> MFLIHFVHYKTILQKYTFKFKHIFLSIDKYNSLFFNISGILIWLNIIHINIILIKYSFFILINNFEYLIILIST;> MQKLLSPRTARHARLFRLAGKLADSGSPGVPKSDGERLVWVNSHVRRDKDISLSQEEERIRELMMPLEVGENSFAANGQATHGNLFYFREYPMYPGEYVPAEHNTLSSLRDELRLDLTAQSLKEAWMRVSGGVYFQSVDEYYASVDGLDAEQIGEVLAALFPELNCYEAQALVQRTLECISRPVSAASRQLSRTITAEAVGLDNAPGHYTNFLEWMGRLTETRAFKTEHALFEFSRRKFNRDDVRVMFENYRLMSKATLLADSADSYSHFYTVLKDFAXKVAGEDSRHQIGVRIDEAEVDPETGIAVGRGCADGEKYHFTALLRENRDHNGIITVMGKPLSLVLDNKAWLMEMVLMPFDEANLDYRDFDAHIVSEGHAMPSIANEIAAFALRMAVANALVKLIPLTRIPLKKSGLLSVDRRRERGQFPGYLDGKKVKRRFAKR;> MVRRSHVVAYYWSRYRMPTQMPKFDGPAPVAAPQSMNSTKTNEFIDPIDDKFPMSIRGPLVRPDVPEDQYVDSWYICTSMTHHMGDYRPWSASAPPNAFRFRPFNEFDAKGREYVQYMREFARFDPRKSRGNGQKGFPFRDAYLTKMNEANQKTPPPTLETIMDRAVREHHQHARILSPLEVQRDVGRLEPIPSYAGKINADRSVFPFQWKTEDWYEYEVAKVRNRRFVFENTEEDGIRGSEVTYKIVLEGFWDHHVMKLAEDVCMFLKDVGRQIVEEKLVAVRRLLQGGAVDPELLAAFNCARAGPFGGLDEYDKEEVANFLRSDLRRLEEQCLSVINRCNVPVPGATNIYDPHTSWPHVEKLEPWVRMAEFWTSSSDTSFTELEMSTAHYEFRKFFRVIICKLPFQSTEFEKRMYDIRHWLHRQTSCEFHTIYRRNVIHDSAVFPTEHDPATPTTHEHHRMFSFALDWQSAPVNRLSTDTVHEGESWDAVAQRLGCSVGELKDANAERETIEAGVVINVPVTATRRLTSFGATPLVLPLKTTSAKDGERIRTWEEAAAILDCTVEELQQCNGHAALTYQKKESEAGEFDSSETELVAPLSCWTSTSESEFSPVERVHANDTLVAIARRLQCSEEALRAVNDGITDVSGLDFVRVPPEARRPRRLVEPQLRPQAATDALLARTIAEEETFKLKSIPHLPQNAERFPHEYHTPTSRFPPTPSETPATQDWMAYTAKYLDKQFTISAEPAPVYNVNKLWPMQQIPGKVDQTPFEEDQTWLLHSIPVQQLEMHHHEKDLQDLPFINHEQFPRSLEWNAP;> MMRKSVTFLRRGKPRPRAGMFPDKYRRVPMLLKPQQGGQQYFNHFLIRSTNDRLTQQDVDNASGQAHSFISPQLPQMDWRNMSARSSEESIREEMRQLAENDVMQHQRVFNERMWYEKEEEHRMKARSCPEETSEHAXSNDGAVPPPRVLGGDYFKTRFGYSLVKNSEMTQGPVDYSQLDMWGEMPRYTSDMVFLYLVSRRRNTYAVAYTYEGKRILNTYTAGNRGLKGGDRGFRSEGSTDNGHQVTSMYLNDLLPKLREMRASEGRPMGRGEKVELVVRVMGFYNGRQGAVRAVQDRANEFHVRYFEDITPFPLNGPKMPRGVFK;> MFCFSRGLWMRHIGQDVPKRHTHFVLESRLMYEKSFRDCWLHSVCRAISQLDEPLSKTVVGTHQKMLQRKVTCFQYNQYGLFKTPYYRLANVDRYHAVQGVAGTREWVPYVNVSYWTMNKMVRGGNLLVHRVHYTGWGTDSHLKKGGWEHRWNKVLQRNVLQYSRI;> MNRTGGSIYAHALSQFAVCRQPWNEYIGLLTKQDSTPYHTEPQEKPAYRGRK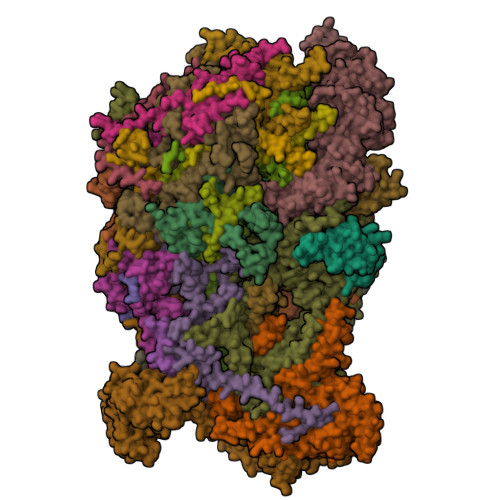QGREGWLFGQQVQLHYHRFPDEQLITNLSRWRTGETVGDIAMQQFRNAQPFDIEDKDPQGVQRPSPEVYMKLNYKNPATISRFLTRTGHMYPADILPLNPEAVVKLRVAKAQAIRIGLYPRFGNPFWFRSQKFRPKAYQENYDPTTYSTKRTVEHFAYNWVQTDRIRRYFRELEAVHTSGSASARGSGGGTTAEHKQQDQFYSPENQPISLHRNNISYMEDVGRSVKNPTVPGLMSTKGMKKKFHNLYSSTSTKRMGFSNPTLGIKKV;> MAFRNTFTTPGKFSTVSKNIVLLLIWRVKVFLRAEGFAHSLVMLPVSLYSKILLCDVKKKIVYFHCCTRKKSMLRRCPCVWPDGPTKSSVSIGTAFTLQKRFLKIAKSAFGFYLARRGQRKYPFLRRPHIKNTHSMNPSAPYFWSFMTAKSQMAFLPEENYITGDWTGKFFVSKRQVYTLQHATSGAKVRVKSFPSIFEFNSPSRWNIGKEMNTLTKPRMDLIDEQMLTKKQRLDYVRAGLLPK;> MRSKTLKKSLAAMYMRPPVTCYTDACEAPVAMWDGAIPLKETRKLKNGVPVRTVSRTYSHPPQLTPTQLSFNDINSMYCVGNDELIQFFPEGLGGRVFQTMPPGHPRGFLYRKETHLLNLFVDKVQHWHTKRSVLSSLTNGRTGFIVDGPTGCGKSALMCQVVHFARSRNIVTLYVPDAKVWTHGEWCWPSTILPGFFDAPDAARSFLKYFAVANRATLTSWKLRCTPKDLPTEQGERQPQNLYELCEWGHRAVAPASIDRQSVCVKFLMDELSEEKKLPVVIVVDGWNLFSHETHFRYPHPDFLRGLASFNESSTDIDLYPQELPRIPASRLSFVRGLNKMILSGDDPNKFFITCTTRDFKPFDGISGFPNVETDRFANSLDEYAPYDPEKDSHFHPIQIGNFDEYEYRSFLRFLINSGELAGLGWGPLWHASSDFERKLYKIGFLSGRNPQGVVDHYHQELVWRYDYQRTRQKQYLLKRRMEGMSRGASSGAVGVR;> MVLRRWFPLLGVHRVGYTHPSTLPVPCAQRWDLRLARARIFQEYIEEKAPGAWQLEDERSMSPEFKTFTGYPMRDMRPGYGQNLPDYIMKKRLPNNTHYELFARRDIPNEDNAMYGKYLYDMTVHGTSLPSTYRMHKDINKAQRNDRKLSGNRFKVLCSSGAKNPPSGWEPIPDATEEEED;> MRRWHRSLNPALFGERGSGHYFSTTRARLQLQAQDRIICGTHGAGIVAHQTAVNSSDNPMLSSVTTAAPAADLSRTKPHEGTGTSERDPYIRTLHNQRSAAPESSVSQSHTVNAPTVDECEMLAERWGTMNYWHNDTFPRLVVFLKKLLVPDVSPLSPTAESLLSMFEKVVIPKLTSDEEDRRKLVSLWSETTLQAEAAVTKFLFQRGSFESMLHRIITDALEKMSTLALGGQEGNLALEALKRQTLFKRNDYIQKRLIDVVSNSAYLGYGDSVWQVFFAAVEANEENLLSDRATTDAIRAAWEGVMREDVVRLPDVTGVVALYLTLVCIRESGRLVPEELKELSSGLEDGVRPGVRKLQQYPLIFLHPTVKRRFVVKAVAEILHNSSSNAFSNMLRENGLHDTAREVALCEAMNRNKELAEGDVGDAVGRFVSKGEVKTLLSSLVSGTDAVVRDAVAGIFGIGTTITIDWDAVMQNVDWSNNWQRLATALLSNSAVLSAIVKLVKNAIGAKGMSKHLFTDEYADQLQLILDAREERAASRKQRIENIAQELSSFERVDLSCDLLRKLGVDMTELDTAAAATRNMNVVQRPCIEDGLLSLVLEAVTKRHPNWVKAGVIQTTLKDPFDALRWMMHIFIRLSYVPHAGAATIARLSRRRIGPIGLEPHQFNVPAELGFVEQYDNLQYKRYDWQGWYQRMLDVHNRNVSLRCRICDLQRLDGNGVQFVDMQTERRLRILAQHRVGMGVLKLDADKYEDQADNVTFGTTKLSELLADARKAQLGEEYWPSVELKVRKPSGQSKAHYSLIDNERIEKRSRELYEKYRDAKKRSLFVTPMETWLEVKGMQVRKSVDNADEDGYTLDALQDMMDGDDGDKV;> MMRRVASTGSNGGHCYVGSSLWADSVYMEVSSITLQKRFSFKYATKLQHDEMRQPYYIHEKRYGIFSNERNIAKARRGLPFITPLYTKHMNLWDTDTDASNNRFFRGYYYGQRELHQLLGRPHSLEATNADGSNDLSTYEANTSQLYKGIPRPAITNLHYEPAWRYTLYQAGAHGAQLSNPRSPFTAKVLGDELMQVRDIKSVEHCKAWFDRLQYLINLHYEAVGDIGEFKSRHTRHVHEFFVAFHDALSSLDFRDTYLFDQFKAVRPPELSDLFGIFLEMEANYVHEDYCPRCSLPYSTTRYCGEGDVDTPFRKHRGRWAPHQKWGREWYDVVARRAEALWYRATEDPYFGTPQHTQRQAEALLKVYVQAKQRGKAIDFMNKLRGSVEYLTGDITITTVMQESYDALLDTTPHPHLLTNGFTLESDAAKYTGEVNKAPLSPLQFRIDMEMNKYRRQQKEEGVVRVPPALWRLDTSAIVPYKVDSKTRRIVNWREVKEGIEKSFLSVGLPKEAYTGNEWREMLYLHDVIANREAKAAVLEQQQKLDREKLKARERASLKGEKSSNSASNGIGIIFPDKDGYQVFFVDEASLRPFGIGASGTLFKAVARVYPSPAAVPYDDPVHGKQFLIDTTDETCHLFGGFEHGDRLLLRAKSSGGDVDGGNNSNCRNTGSFTDEEEEVIVMGVSTEGSDAERMLCAMHVDTGKQRERGIVFLGTDCIDIRERWESVRYAASAYVKGRVTLLESQRTAREEFMGQVVGIRDGVLFVQWRLLKGGGSVLDRSVAVPIGDSTQVRELFVETKVLGVEPLQSPPSWRTPFRNDFAEERLKELQRAPFKREKYVSLIQGKYTPKVKKFGYTQHTTVDDFETKEYKDRLLSKQFFQNPQAFEVVPDRHERSVQFGGKWEYQRTHGLPTVDRNELENGWSEVEPISDGEMKVIEQALRDISGPRPGNFVKPPSKTKSLQLSESWWEPLGYGWEQHNEEQKALCDVTEQRLIDGSNLPFGGKLPPFGTSYGMGERMRAIIEDYSKGFGLGPHGHSPTHDTIHYNTLNAEGERVRDLGYTDALGRLFSEKLGDRDVHQWAVESCADGEADVRQLLLSLHEWRERGRPPSLLLANVLSKYLEEEIAAFNKGIPENAPKLQLETSDGTLAHSGSGGSRSGTMWADVDPTTFALHQASQSTRSTRCDEPFILHLVKRAKLGECVTNFTDTAYIAHLESSVINEFHLALTKLVGKGISPTLLAQKTGQLHRGSVRVGGNVVPFVKSRELSRLLERMGLTSESIAVITRGLANCPEQESVGDDFAVPVSLILSWDGPGSSGGSGSGDRRLNTTAARNEQQRKGSAALSSAIRQLSQHQKQRGSASGRGWQNEDKMVVHVLEELSLRNDGLVMDIQYAIRENKKNRRLRWEFVTTLLPVFGGNEAKVEQLYSDYCDGKYVPNITVAVEAFIAFLHNATQHPETYSASDYFDIDDGKSSTASGTGDQPSAGQYTTLKLLDPLEGPFVFDNVKVEYIQTVERFRRHGIRAGPVMAPATGFIAANCKSLNYFTRRQEEVVYVTNDSDQGLRRSLENSAYHKTIAANPALQYLLKARRGAALVETFNRFFYRTMPMLNFYQNVLKHYSETIQPLRQAAKSSTRGLARALESERSAAMEEFRRNSERYWRNIIEGRSVEQVVLANGESNRRTVGGGAGEQLQKPQGNRDAVRTNFTGEATDGSRKGQRQHQQPPLSQQQQHSRGEGERSAVHTSPRQGGSRGMADLLSKLNTPKTGSGVKGSTAKNTGNNRRGPKS;> MIRRRVCDGARLAPNIRATFSAVRYQSGLHTFIRDSKPSNFSSVRRSENANGDATASPGATAGENPASSGDWASHMQRELFGEVDPLGGQAHKDYYRDVTRGYSPQYAPRNFANGGAVAYPHIQSPYEYEEAAHRRVWLDHDVDRMREEFTQHRASLRSLASAQEREELLRSRAAEYQVANTVHESESVHPIQQLYNSGGTSRSALKQQAVADRYSIAEQHSPLPLTTGVDRDALDEAQRTKDRILNDSFTAENLLITHGLREKEKHDFTILQRTVRIPFQGYDMDRFLAQQKGTPYGAQQLPPNVVPSSMEEAQRTLRGSSATATPLVDAVAQKVYARNTVVDRPAIGEQLTEQIINIMRASRTTAEQQREEERAQRFGLGRQGALVQDGGPDQRTLKKHTNDERIVDAMLFQQNAYRKTPTDEHWNPYIRRSTENGVGHLLQNKFDIMRREDRLSKGEQDLTERNTIHYGVPIQQIVDEFVFRHRNARGERPLDYFKPFPNFRALRLNRMYRDVEGFSLMKQRPEFLEWELFTRYRQHHQQRRRLALLHGLEPVANETAQERDTRRHRLDEICERTPFDEREMRVNDDEMRVSVETLRSWFGVYMLPSPTVVNAVLGGSASVNLHLYHLADEMGTADTREHVLSSRYLNRLLLLESYQNRVGRGFMNHVVGRAPEPVVPHEQPQEVLRHFSAEERAMYEQHVKEQTSRQLGEWERAMKRRRWLTDHQQYGHVVSHGLETSVVDLSHTETGAVLTVSTKAYEQEIEAVRMKTNATIKVDGMVYNLLPNSERRVVPLTVQLDSGEKIDMTSEDFDRCELEAFPRNLNHALNYGIANYAYNRGNYVETQDSIWEEQTASGQEGWSPATHADGLREGLPVRARRPIFSSSAEQRIAGGPQRAVIIQYHHQPFFNPEPRLVKVAFQCDGTIMEVPISDVMIWQRRYHGPERTVGDESRRYNPAAMRRYVDVTDPFNEKTSNTEHFLDKYEPKRNADTVADKYRTTKQITEIDKWTRYDSARADNYRPLSISHRRDYIRMGYIPRYTPWEWIAIQEADQPLIAEQIRQDNIGTSYFFSLNRYWRYKASPHGYIRHFENEVRDLLQYVDGVTPWKQAQKIRTYWEVRSHHPMPQFNRPEVAMHRNTVGLLPAHMWETDKKTGKVKSVKDSVRDYQTKTPYPKWVQL;> MFRVRRLAGFIQCSPCGKMGPLKQQTRRYTPIWKSDPAVDNVAPLRDEDERRALWAEVGPISDVGSAVTAWIRFGNDPVLHTAVPTMLGGKFRNQQREKESLLPNSSSPFAYVEDYMGTNLVFGSPVHAKESAAVWATYFERRYASRLRLSRRTVANYVGLINSPEVFDDESDRPETRWSQDTFFRECAYLSEKFLKEKVSNMQQFEAALKRASPEAYLAFFDAFQQQTQTQIPLPSPSVWHYEGERRKQWAEKFISISHKAQAFFKDVLSEDVKKYQEVPGKLLQKVKPVLADVGKILVKRHERWLKGRVWTSLTEEEREAYCMKEVKRQQMQVEDGEFDPMMEDDVDDTELEEWQREHDAIMKLMNSPIDGLHFTTLELWLHTMRCEELETEHIYTSARVRAIQVAARKKLYDTTSYEEVIQAVVESIARGTLDLGAGVLRPHFNEVWCQLNYAKFGSSTITQHTTTSRRQLLFFHAGSLKDIAATATLYYATKPLSNSLDYASPYKYRRSLITLCSNYGVETAYTTQRPLLRSAANLARAEDLIHAVVTAAAQPFGERRRAATRDLHMEFQRLAVPVERVIVANPVSALLESGADPDEKPVEGEKVNMWPLGAKRVVLYKWSAPNVEKLKAMESDAASAVSGSSLTAKRLREIQELKRRGFLEVSLWRRVTAQERKQRNEIVEAKKKQVEEVVRTVPSLAHLHQYATSLYSRIEERVAFPTETSTVTETTNMKEETNKPLEDSEWEFAVLLDDRVLLNKEESVELYLPYRDANGELLAQGEYRALVRAFDLEANPNLHPAYCSVGYSESFQVFDALPQLIAQFFRVKDATAEAAGVTHIPAADFTPFCAFLRDAGLDVPLRCEFEAGQAVTTDGDVYMDYFLQLLRGEAFHQSHAQAGLTEAQRAIEPLCRAHWVVHHPGADESEWATARRSVLDHAMQHEREWWFPNEMLDVKDVVTGSTNGLTPQMYPAAVRYGVELCTVLTAEGKFVDERGSGLSARCVVNGTGAAESVVFDTANCNGTNTTSVEDALRVAHGALRSAQDRHNTLAAFRLGPLSKQSQVLLFCGVNAYEFGGKYARTYAYAFEKAKKELEATAASGFMAPSLSHEDTERLSDQPTTSPSVDRFASTTHPEQRKAQFVPRVGPGSTPLEDPAADQKSEWS;> MRRCSFASTCRYRSADDVPLGLGSAYVWTCRNITSRGQFNPIHNFSYAMERGVRARDVKAFEKLITNPGPLRVAYTPDYLDWLHRCYKAKGTYMDARAVAEKKFNGNIVSSELSAAVNRREGKRGDTRGDTVDNDHHNLPGAPPPGMFLRPAHSFRRLAGELKRRRAQSILDEVARAQGMLDLFERQPHFPAIHIDRCSRFHLVELFKEMVLERSLDSNMIWEKALLYRAILSERKPSYPTSFHYIFTAVEDTVFAPTISTPMEMAGSGGEGHDRSSHPLAAKCPTLEAYYYYVYLVKKYYIDNAVEAHVVLRCHREPNAADLLFSNPPPKDDTEIMKAVELLRNADIQRGVAAAAAVSDPTLPPGGEGSVIGNSDNKKNSEKTSEGSRGRPARPPVLPGAYPPIDMLWRCEENLPLLKVLLFGEFNLIVSENPFVKFPSAHGFLTRPYSTDSSRTLADGMSLANVMAEKRGHLLPSLPRNTATSIDARAQDIRRLQQKHHRDDIVSFQKLLRTTHAEDSPSAFSSYSDWSYFNPRAVRAEERDRLTRKAVEALKLYDSATNDIYRHSFEDVQACHTQRVTERDRTMPPYLPTLPHFVAIIKKDPHISFLLHIGLPDRNSSEEGSAKHKELEKRIYYLARALYHTALEYHNETVRRVNRQKVNVAASLLDNFVEQEWTTILRDKHDVTDVTKTLNDTQNDKKQLARRLGRYMLFANRSLDDTGFPTDARADDYTRWMAPPSVGKVSL;> MSVSGVFSKGRGIGHEATTSILRYIPRARVPWQPSRFGRENLTAADMARLWSRGRYRDGPGNYNSGYCTERTHVLEENTVSIIPRRELEKYMPDITIGPKALVTPVSLMNARNGHRVTHDLLHSYDPHIGRLGKPAVVDHDNITVEDPNRVGLNAATLDCRGRIYRWLRRGPFFQVDNYFRRSVKLNRDGTLPTDFVHEAPLMRKIIRLAHRGHLKAACEEYRRVTTVPPVEVYRALTACCVPGAKLADAVSIFEDGDSKLFYVSRDGEVLHNLMRCAIAARHRARIMWVYNVMRGRFYENVVVRAEVDLIWRYRIAMIALEYLLDHECAEEAAAIYSYLVEEELLRCDVHVRVGLHMREAIAAGKPITLNNDVMNATSLVRDATAVAPEVARELQRRHAQTLQNNAVEAVGAENVREGSAPWSILGPLTAIGPTAEDTMVWLQQHYGDVDVMSIMRWARFRKGKDLMAKDRPQYLARAAAWIELLSKRNREMEEVPLTYMRKSKPLVLDTNSNVRVAWQTPLMRSGGPPRLLAREEGYVFHHSNSSRFVEETYRHPGESLQSRYLALQPLHTEVSAKEDFQRLYYQAQKHHKQQERLLPVSTAAIPSRIVHHSVMSALHGVSGKGEPANRSLFTXNKSNDSHSNTGVASGTSACTDGAGSATPEF;> MFRRAIPLLSANIPRSVWDPAQHNPNWSDSYGHDITNRRAWPARKWTVGLEPCTPREWLQFSHRNLAYAYNGALRACHSLPSMLLLYKEMKQRGVKVDVDTMNVLLTRAARHEHIQVDDVFLLFDELVALGARPDLAAAETLHTVLSHSASMPEEWREARRLQLVELYNNLAMEEVERLAPHRADRLLKEQMKRFRGNLQQLGSGLRPTVYCRYLHTTHTAAVLLEEVHNFLWELVPNDHPAMEIPALQLRVPFVASVLRRPSVNPGVSLASVSRAEFGDTDVCAVFLAAAERMVDADFDDQRPVSERRLFLSLLTMISYSGVLYTSDLMAQLMEMVKYSNNDETRDSDAQRVLRYALRGSSAAQDSASRTLWHSVEKVADCRVVGRYIGARNPWNPIRVCFDEQGVFKAYPISTTTTTREVSPPEGNGAVTQEQRASCVEGRTLEALNMRWDDVRRLIECTGVLVTPPSERCPQQQKMEVFTGMAVYLRTVATGRRYEGGEDVLSDGAVATSSCEQRRRGTLFAEGYDFDVWVRLFSLVQEVRHDMEKFMADHTLQCVEPEFECWEALLVTLRCALDFCVVQMQGGGARGTEREVVERLFRDVVALREELIEESRTRFGGRMRVLWLQEA;> MLSQNVAKTTVPSYYMIRTNLPHRKPQNQWEGVYYYSGITKRQRHLILLHRKREREAHMRSFNISRASVLQRLEQLSGDRKQESLPPHVRLDLAVRLAQHGLYQQATPIVDELHHQKALHAGHYALLINALACPRLGQRILHCDAQCDPALTYKLLGDENGEERAQEAYRWFDLALTSLAVDCGGRTQPSHFVPYLPQGTAAASHITNALMRTLLTCGYTHVAAIPDSVYDRMGSMGISPTISTYELVMLALSLQGNMVEAESILSFLRSHHSEHITVESFNALLLGHREARQFDCCDAIWQELVDRRWPRASPLTAELYLRSIMDHANTPTSEPLQSFANINVVEKKKVPLVLAQMDELGVPRTHLSRVLMDEVEDSLRKFQTYRSRFYEWGRAVKQFDFIEFRRRNGWLYDLHLMKCTTKQVGPLRDFNDPDAVQGAVATAEIPAFFNERPAWERPPLEETLYVTTNKERYDDVRGGDIYYDDTRGLHDRSPTWMNEVPETRYDRLYGVNHPDIAKIGIRRHLNVEYVNRKEVVERDAALMKKTLSSGRRLRHRVESSRTHRNAGSLSGISSTAGGGSR;> MFRSTRPRSVGYTPVNPDTSPMVAYSQYHWHYNLPQGMERPHSVNRTFAAPFQSNHSLVNKYRGVWIEFDMHPAFSVALEPQLRKLPRGRTLPKTPAEEVIADYTALAPLVDDEKTRDLWLAKVFQHCAFQRCGGAMELWERYCHQRFTAEGATAKPPLSLVKSVLFYCNKTDNSGWRALFDRCLKDGWNYTPLFDTAQWSFMLKSIGRMGDEDGVRAVLEEMLDVQADLDRVEARSVVIALNAVTNADVYEFVKKYLFNFGERKVKFLRTTYSDLRGHGAGKLRIPLKENDNMYYHVCWHSSIRSPRQFSPRQLYFDYTPSTLGSSSHNPNAKIDDIVKDKIEKWKAEGLLPEDYVHEDRVYDRSAAFKNVARQEKWKKMPKILKSKRMGYTGDP;> MSFRYTNNLIGALKHRLLLESSYREIASRKFIGNCRGVEVVCSGYGTVLAVQLTDKAVWESFYRKGGRPTVSGGGDVSGDAETGTQGSATTTGATGSLDLDKLAESIKTALWDATRKIRSAKEAALHRSLSHNTRMRASADLKHWYEEDANTLRPLAFEALKHEAATPWMQLVQHGKKEEAAALLKEFEQKGDAAEATPTRVKDDRVKGTRTELSNREQPPLASTLKAEDSNPATIPIGSVHPLFTPALVQIEEAGGGSVSNEAVCRAQLWELSRDEQLFWERVELIRKGQVASIGSSHKRGYADEAAFAKDDTEEKVQLRFTQ;> MRCSCAFLDKSVFAAKRRVIVPIHPTPNFPAHFIKSAFTTDPLKEKQKARFSSGGEAMREVQDIPKNLEGERSRRDLASRGDTEFQALVEFIEGASYDQLISGRRFKKVYDVLSENDDMFIWLCHTAMSVLNPGDMRSRLIYNHLRILAESVASGEMTQRTAFRFFESAVRSPAYREIAKRQLEGGAATRLAGISAAADVMRRMGLTRRPMSSYFELYQRIVERSEAMTPWGFPPLFQFEERLSLEPRLKFFSRASQQSLERRRRGHVMTPHTTLHGRRIFWIPPTWNRAGRFLGPHVTLYPGMTPD;> MLVSYLRLQADRRTRHHMMVDGQINPREWFNWHPKEYQPWYFDRHKFLYEQRQYAQFHHLLCHQVYLKDMLHLMRYPEPYTHIIDCRTSTQKMHRWVPHSLWLPRDEVEYALQLSADEFLDMYGFRKPDKSDDVILLSHNGIYSEQAGWEWKKQFFQHVYNYRGGTNELFGESYSDMNVSDVLSPWKGPFPQSGVFVDKWSKRKVLTRTGPFDRQYEMQDFALPDLELEKARHPEEGPRQNMPFGLQ;> MRRVRDGLFLSHPSSALQCSVAVVSTGEFDHPPFQFRQRHTFNTTPLHDANRFGGRTAYLREIGPVNIKKQGRRFKKDPRTVQFNVDVWCAQQTLRKRWKQRDWEVIEIPFRLVPREQQRVIPELYTDIPQMTDPARNDFSNIRNKVYDREELQGVLFPAAGAMLYPPLQRVDKQAMTLDKYL;> MLRFTHRALTATPERFSVLGTTHPKPKRTGFGRNNKMRSKPSDNVAWYDKGPVEWLPRPVRLTYDHLDQLQQWTMRATLDGRTEEFNRIRDLHREWSQHPLMPVLGDVEPKFPLNLFKQNHRAKKRFLVRWHKANTPANWLWMPRGPTVVTPLHRTNPTQYPENWKQMVQRKSGTGTPS;> MFHRAFVSSSDLTGCTIALSSVCTQKRYWAKPKKRPKVGQGFHEKAQKWREEYLLDRHRALADSLRAYVEFSTSKRVEPWDARFKPFDRIEKDGVYVLMRYMMEEKLQLCNYHHRPVKRLFCNIGLMGPQITTKARWKPYRFATNPAGTSKAERMYQRDKTVYTHGHND;> MLRSTLTSLNTFLTSSVATPPISVIRTGPKWWADPERMVRQKLMYFTLGVDQLPLRRTAVIQRDLQRFHMCKPPPRVGDSTGYKRSRAAQLNTWYRRIQYQEYHMQHLFTRHVWGLLRVYPGNTTKIQGKADDGYVGYDSVPFHRYNRAPLPFPARELYERRK Based on our previous studies, which demonstrated that hQR2 could reduce a large variety of quinone or pseudo-quinone compounds, we hypothesized that hQR2 could play a key role in the bioreduction of these indolone derivatives, because they were pseudo-quinone compounds. In this case, the indolone derivatives would act as substrates, not inhibitors, of hQR2. In the present work, we demonstrated that the anti-malarial activity of indolone derivatives is linked to their ability to serve as hQR2 substrates knowing that QR1 is not expressed in the RBC.

Indolone-N-oxides (INODs) have antiplasmodial properties that target the asexual blood stage of Plasmodium falciparum (P. falciparum), with IC50 values (drug concentration required for 50% parasite growth inhibition in vitro = IC50) in the 1 to 100 nanomolar range [4]. To confirm this interaction, we co-crystallized hQR2 with the chosen substrates, and subsequently determined the corresponding crystal structure. In this case, compounds 8′ and 10 were selected as representatives of the INOD and IND series, respectively, due to their high solubility in DMSO (solvent used to dissolve the compounds). Crystals of hQR2 in complex with flavin adenine dinucleotide (QR2-FAD) and bound to compound 8′ or to compound 10 adopted the orthorhombic lattice conformation (space group: P212121), with two molecules of hQR2-FAD and either compound 8′ or compound 10 per asymmetric unit. The ligands (compounds 8′ and 10) both occupied the same region of the protein; both were located above the FAD and interacted with the isoalloxazine ring through π–π stacking. The ligand residues could only be partially modeled in the electron density maps; in particular, no electron density was defined for the terminal anisolic ring, likely due to its flexibility and exposure to the solvent. Compounds 8′ and 10 did not establish direct interactions with the protein residues, but interacted with water molecules present in the vicinity of the binding site. The structural data clearly showed that these compounds lingered in the catalytic site of the hQR2 protein, comparable to previously obtained data on co-crystallized substrates and inhibitors of hQR2. The water solubility of these compounds varied strongly from one molecule to another, ranging from 10 µg/mL (0.33 µM) for compound 1 to 1–3 mg/mL for compounds 8′, 10, and 12 (3 to 10 µM).

>MAGKKVLIVYAHQEPKSFNGSLKNVAVDELSRQGCTVTVSDLYAMNFEPRATDKDITGTLSNPEVFNYGVETHEAYKQRSLASDITDEQKKVREADLVIFQFPLYWFSVPAILKGWMDRVLCQGFAFDIPGFYDSGLLQGKLALLSVTTGGTAEMYTKTGVNGDSRYFLWPLQHGTLHFCGFKVLAPQISFAPEIASEEERKGMVAAWSQRLQTIWKEEPIPCTAHWHFGQ[2x]>[10x]MSLVVFPFKHEHPEVLLHNVRVAAAHPRVHEVLCIGYERDQTYEAVERAAPEISRATGTPVSVRLQERLGTLRPGKGDGMNTALRYFLEETQWERIHFYDADITSFGPDWITKAEEAADFGYGLVRHYFPRASTDAMITWMITRTG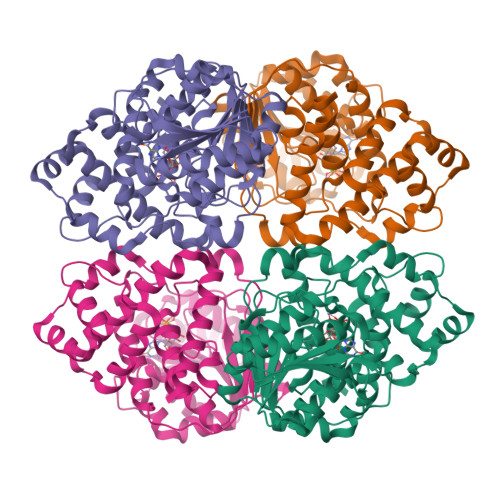FALLWPHTELSWIEQPLGGELLMRREVAAMLYEDERVRRRSDWGIDTLYTFVTVQQGVSIYECYIPEGKAHRLYGGLDDLRTMLVECFAAIQSLQHEVVGQPAIHRQEHPHRVPVHIAERVGYDVEATLHRLMQHWTPRQVELLELFTTPVREGLRTCQRRPAFNFMDEMAWAATYHVLLEHFQPGDPDWEELLFKLWTTRVLNYTMTVALRGYDYAQQYLYRMLGRYRYQAALENGRGHPVPPRAALSTA> MKPPSFDYVVADSVEHALRLLADGGDDAKIIAGGQSLVPLLNFRMSRPSLLVDINRVPGLANIRKSDQTIAIGALTRHAKLTTS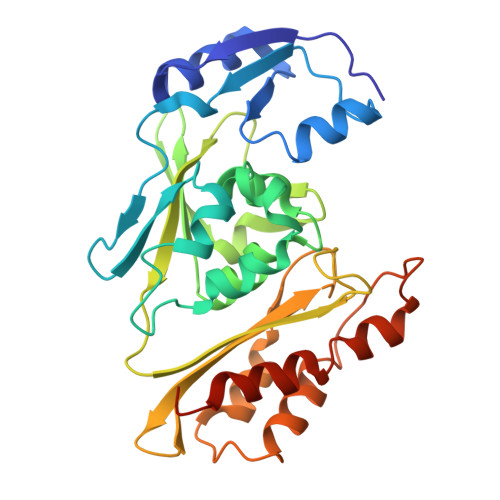KTISQNLPILSEAAAWIAHPQIRNRGTIGGSLAHADAAAELPVVLLALDAYVTAQSLQGERKIPLKELLVSHFVSSILPGELIVEVNVPQLPHGSGAAFDEFSRRHGDYAIGGAASIVTLDEQGKCSRARITVLGGGSTAIRCQEAENILIDSTLSSHDIAAAAHAAVQGLDPVPTVHGSAQYRAQVIRTMVERTLAKALHRARPTKESMDH>GSHMASMKKKGSVVIVGRINLSGDTAYAQQTRGEEGCQETSQTGRDKNQVEGEVQIVSTATQTFLATSINGVLWTVYHGAGTRTIASPKGPVTQMYTNVDKDLVGWQAPQGSRSLTPCTCGSSDLYLVTRHADVIPVRRRGDSRGSLLSPRPISYLKGSAGGPL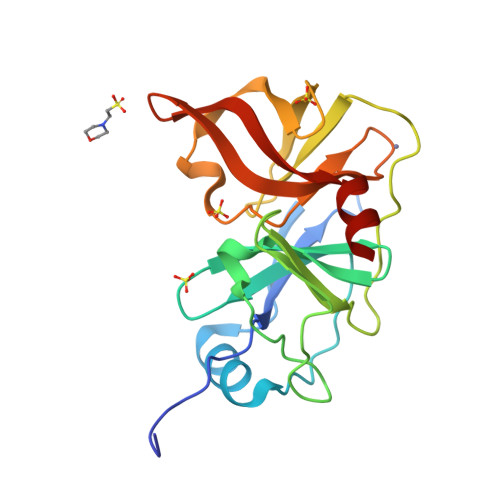LCPAGHAVGIFRAAVSTRGVAKAVDFIPVESLETTMRSP[2x];> XFDEMEEC>[3x]MFFDELKIDNKVDIIGNNVRGELPNIWLQYGQFKLKASGGDGTYSWYSENTSIATVDASGKVTLNGKGSVVIKATSGDKQTVSYTIKAPSYMIKVDKQAYYADAMSICKNLLPSTQTVLSDIYDSWGAANKYSHYSSMNSITAWIKQTSSEQRSGVSSTYNLITQNPLPGVNVNTPNVYAVCVE;>MATETATRDQLTKEAFQNPDNQ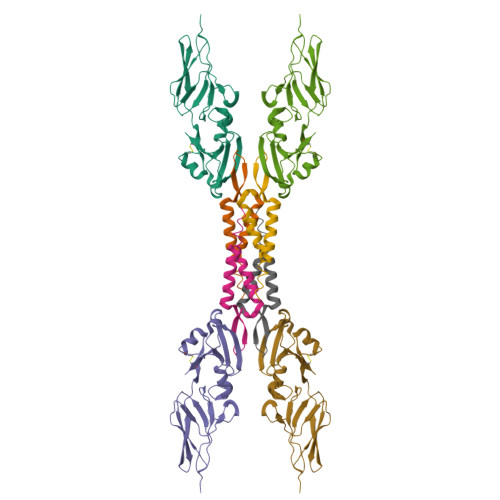KVNIDELGNAIPSGVLKDDVVANIEEQAKAAGEEAKQQAIENLEHHHHHH[3x]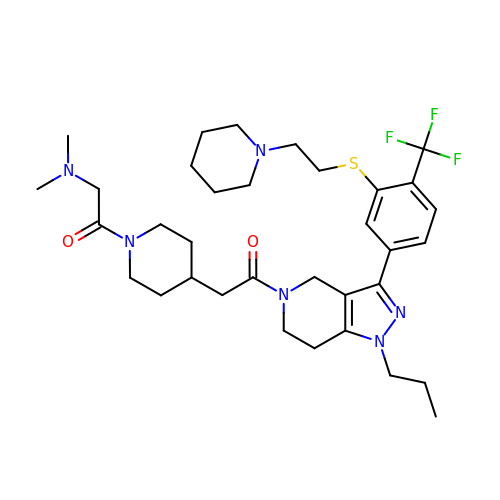2-(dimethylamino)-1-[4-(2-oxo-2-{3-[3-{[2-(piperidin-1-yl)ethyl]sulfanyl}-4-(trifluoromethyl)phenyl]-1-propyl-1,4,6,7-tetrahydro-5H-pyrazolo[4,3-c]pyridin-5-yl}ethyl)piperidin-1-yl]ethan-1-one | C34 H49 F3 N6 O2 S | NUSUQUBVOSMEDW-UHFFFAOYSA-N>MASEAKQTVHTGNTVLLMIKGKPVGRAQSASGQREYGTTGVYEIGSIMPQEHVYLRYEGTITVERLRMKKENFADLGYASLGEEILKKDIIDILVVDNLTKQVIISYHGCSANNYNETWQTNEIVTEEIEFSYLTASDKART[4x];>[4x]MAVEPFPRRPITRPHASIEVDTSGIGGSAGSSEKVFCLIGQAEGGEPNTVYELRNYSQAKRLFRSGELLDAIELAWGSNPNYTAGRILAMRIEDAKPASAEIGGLKITSKIYGNVANNIQVGLEKNTLSDSLRLRVIFQDDRFN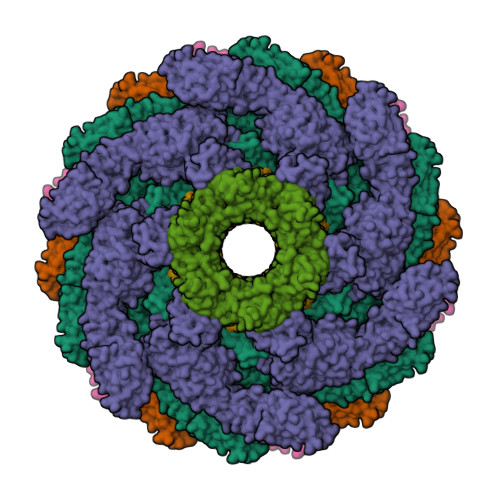EVYDNIGNIFTIKYKGEEANATFSVEHDEETQKASRLVLKVGDQEVKSYDLTGGAYDYTNAIITDINQLPDFEAKLSPFGDKNLESSKLDKIENANIKDKAVYVKAVFGDLEKQTAYNGIVSFEQLNAEGEVPSNVEVEAGEESATVTATSPIKTIEPFELTKLKGGTNGEPPATWADKLDKFAHEGGYYIVPLSSKQSVHAEVASFVKERSDAGEPMRAIVGGGFNESKEQLFGRQASLSNPRVSLVANSGTFVMDDGRKNHVPAYMVAVALGGLASGLEIGESITFKPLRVSSLDQIYESIDLDELNENGIISIEFVRNRTNTFFRIVDDVTTFNDKSDPVKAEMAVGEANDFLVSELKVQLEDQFIGTRTINTSASIIKDFIQSYLGRKKRDNEIQDFPAEDVQVIVEGNEARISMTVYPIRSFKKISVSLVYKQQTLQA>MALEKRNELPACSLKPSLQDRDLITSAEAGEVVVLFKVLANDTRLRLLHALARSGGLCVTDLAAAV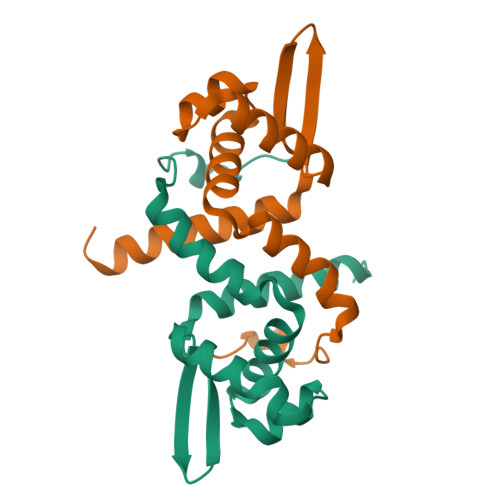GMKPQAVSNQLQRLADRRILRAARCGNNIHYRIVDPCVLRMLELGLCLIEEAEQQAGG[2x]> GDNKGITYEELNPERFTLLEKGTPTNILIDENEDQGVMIAATNLSEDFGRVSGTNAPLIFLPDNERLIIVGTLESRYIKELTENRKIKGDELKGKNEKYLMTVVDNPLPGVKEALIIAGSDKRGAIYGIYELSEQIGVSPWYDWADVPVKPQQNLSIERGSYTADEPAVTYRGIFLNDEAPALTSWVENTYGTKYGDHRFYSRVFELILRLRGNFLWPAMWDWSFYGDDPLNSKTADTMGIIMGTSHHEPMARNHQEWARNRDKYGVWDYTSNQEVIDQFFREGIERVKDTDDLITIGMRGGDGATPMGVKEGEDHLFVSDEDNMRLLERIIKNQREIIGDVT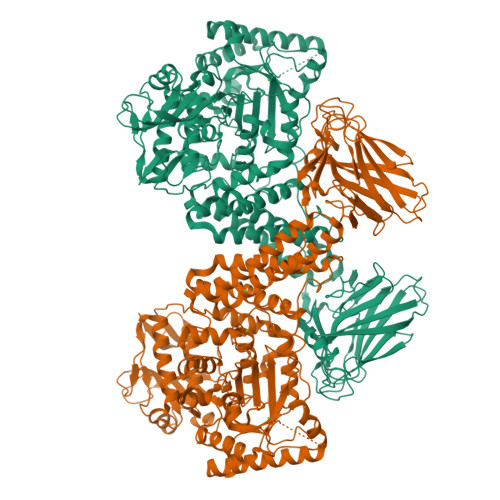GESPEKTPQVWAIYKEVQRYFDLGLRPPEDVIILLSDDNWGNVRRLPTEEERDHPGGWGMYYHFDYVGAPRSSKWLNISPIQNIWEQMQLTYDYGVDELWVANVGDLKPMEYPITLFLDMAWDPTRFNAENLLDHTRSFAAQQFGEDQADEAARIINLYSKYNGRVTPEMLDRNTYNLESGEWKKVSDEYIKLEAEALRQYLTLEPEQRDAYKQLILYPVQAMANLYEMYYSQAMNHKLYRENNPMANYWADRVEETFNRDAELSHDYNKVMANGKWDGMMTQKKIGYRSWNDNFPADTLPQIFRIENPEEATGGYVFTARDGVVVIEAEHYFEAKDAEEAKWTVIPYMGRTLSSIALMPYTKEVEGASLSYRMQIPDEVSEVKVHVVVKSTLPFHDPKGHEYRVGFEGGSKEIVNFNWNLNEEPENIYSVFYPTVASRVVKKDVTLDLHDTDDGFYTLTLEPLDPGIVFQKIVVDFGGYEESRLFMEESPNKRIEES> HKIL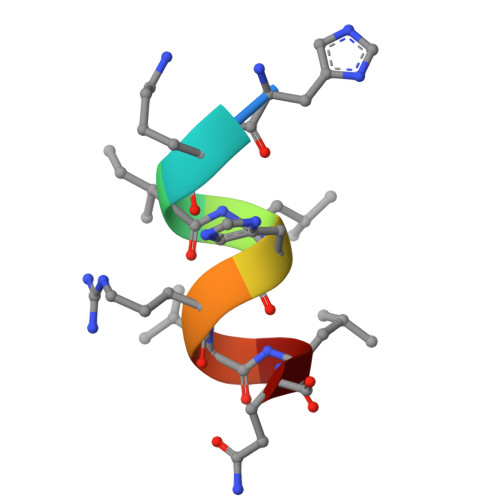HRLLQ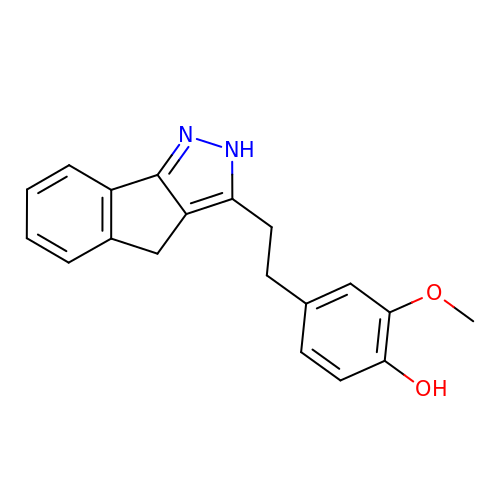4-[2-(2,4-dihydroindeno[1,2-c]pyrazol-3-yl)ethyl]-2-methoxyphenol | C19 H18 N2 O2 | FOIYWUMLZWSWIQ-UHFFFAOYSA-N>MAIAQLATEYVFSDFLLKEPTEPKFKGLRLELAVDKMVTCIAVGLPLLLISLAFAQEISIGTQISCFSPSSFSRDQAAFVDSYCWAAVQQKNSLQSESGNLPLWLHKFFPYILLLFAILLYLPPLFWRFAAAPHICSDLKFIMEELDKVYNRAIKAAKSARDLDMRDGACSVPGVTENLGQSLWEVSESHFKYPIVEQYLKTKKNSNNLIIKYISCRLLTLIIILLACIYLGYYFSLSSLSDEFVCSIKSGILRNDSTVPDQFQCKLIAVGIFQLLSVINLVVY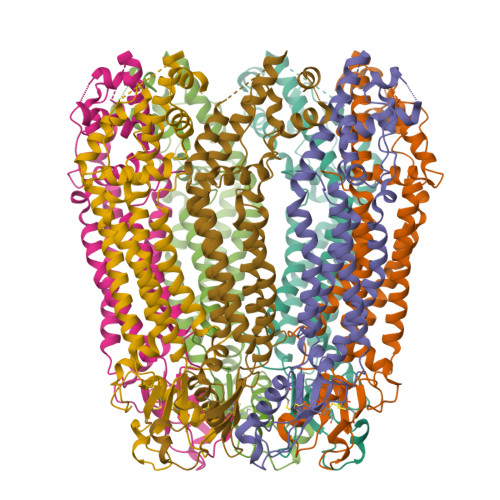VLLAPVVVYTLFVPFRQKTDVLKVYEILPTFDVLHFKSEGYNDLSLYNLFLEENISEVKSYKCLKVLENIKSSGQGIDPMLLLTNLGMIKMDVVDGKTPMSAEMREEQGNQTAELQGMNIDSETKANNGEKNARQRLLDSSCHHHHHHHH[7x]>GAMASSVLVTQEPEIELPREPRPNEECLQILGNAEKGAKFLSDAEIIQLVNAKHIPAYKLETLIETHERGVSIRRQLLSKKLSEPSSLQYLPYRDYNYSLVMGACCENVIGYMPIPVGVAGPLCLDEKEFQVPMATTEGCLVASTNRGCRAIGLGGGASSRVLADGMTRGPVVRLPRACDSAEVKAWLETSEGFAVIKEAFDSTSRFARLQKLHTSIAGRNLYIRFQSRSGDAMGMNMISKGTEKALSKLHEYFPEMQILAVSGNYCTDKKPAAINWIEGRGKSVVCEAVIPAKVVREVLKTTTEAMIEVNINKNLVGSAMAGSIGGYNAHAANIVTAIYIACGQDAAQNVGSSNCITLMEASGPTNEDLYISCTMPSIEIGTVGGGTNLLPQQACLQMLGVQGA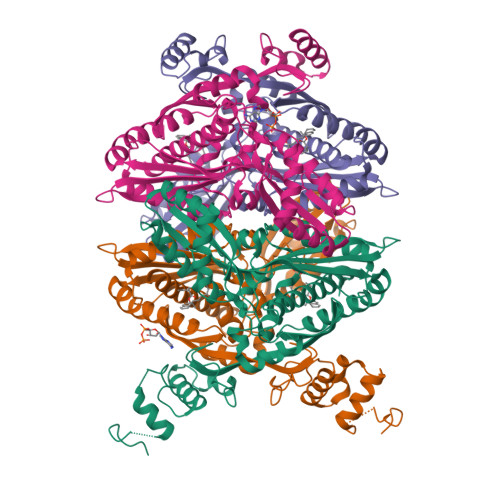CKDNPGENARQLARIVCGTVMAGELSLMAALAAGHLVKSHMIHNRSKINLQDLQGACTKKTA[4x]>GSHMGVKERNRLEAHSSSVRGVAFSPDGQTIASASDDKTVKLWNRNGQLLQTLTGHSSSVWGVAFSPDGQTIASASDDKTVK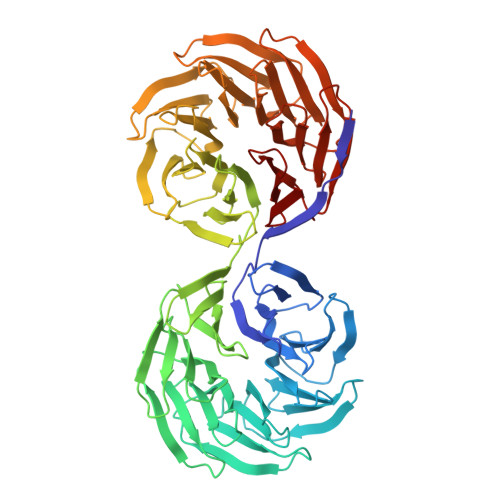LWNRNGQLLQTLTGHSSSVRGVAFSPDGQTIASASDDKTVKLWNRNGQLLQTLTGHSSSVWGVAFSPDGQTIASASDDKTVKLWNRNGQLLQTLTGHSSSVWGVAFSPDGQTIASASDDKTVKLWNRNGQLLQTLTGHSSSVRGVAFSPDGQTIASASDDKTVKLWNRNGQLLQTLTGHSSSVNGVAFRPDGQTIASASDDKTVKLWNRNGQLLQTLTGHSSSVWGVAFSPDGQTIASASDDKTVKLWNRNGQHLQTLTGHSSSVWGVAFSPDGQTIASASDDKTVKLWNRNGQLLQTLTGHSSSVRGVAFSPDGQTIASASDDKTVKLWNRNGQLLQTLTGHSSSVWGVAFSPDDQTIASASDDKTVKLWNRNGQLLQTLTGHSSSVRGVAFSPDGQTIASASDDKTVKLWNRNGQLLQTLTGHSSSVRGVAFSPDGQTIASASDDKTVKLWNRNGQLLQTLTGHSSSVWGVAFSPDGQTIASASSDKTVKLWN[2x]>MHHHHHHGENLYFQGSDVVDPDIFNRDPRDHYDLLQRLGGGTYGEVFKARDKVSGDLVALKMVKMEPDDDVSTLQKEILILKTCRHANIVAYHGSYLWLQKLWICMEFCGAGSLQDIYQVTGSLSELQISYVCREVLQGLAYLHSQKKIHRDIKGANILINDAGEVRLADFGISAQIGAELARRLEFIGTPYWMAPEVAAVALKGGYNELCDIWSLGITAIELAELQPPLFDVHPLRVLFLMTKSGYQPPR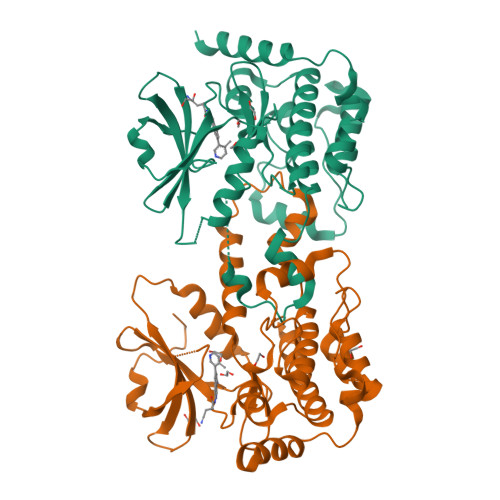LKEKGKWSAAFHNFIKVTLTKSPKKRPSATKMLSHQLVSQPGLNRGLILDLLDKLKNGNS[2x]>[4x]MGSDKIHHHHHHMKEKVVLAYSGGLDTSVILKWLCEKGFDVIAYVANVGQKDDFVAIKEKALKTGASKVYVEDLRREFVTDYIFTALLGNAMYEGRYLLGTAIARPLIAKRQVEIAEKEGAQYVAHGATGKGNDQVRFELTYAALNPNLKVISPWKDPEFLAKFKGRTDLINYAMEKGIPIKVSKKRPYSEDENLMHISHEAGKLEDPAHIPDE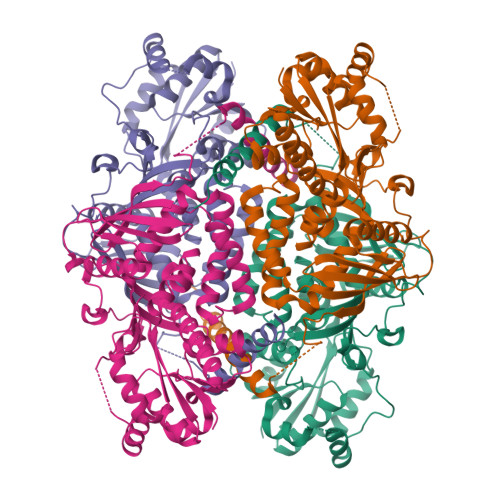DVFTWTVSPKDAPDEETLLEIHFENGIPVKVVNLKDGTEKTDPLELFEYLNEVGAKNGVGRLDMVENRFIGIKSRGVYETPGATILWIAHRDLEGITMDKEVMHLRDMLAPKFAELIYNGFWFSPEMEFLLAAFRKAQENVTGKVTVSIYKGNVMPVARYSPYSLYNPELSSMDVEGGFDATDSKGFINIHALRLKVHQLVKKGYQR> MSAEAADREAATSSRPCTPPQTCWFEFLLEESLLEKHLRKPCPDPAPVQL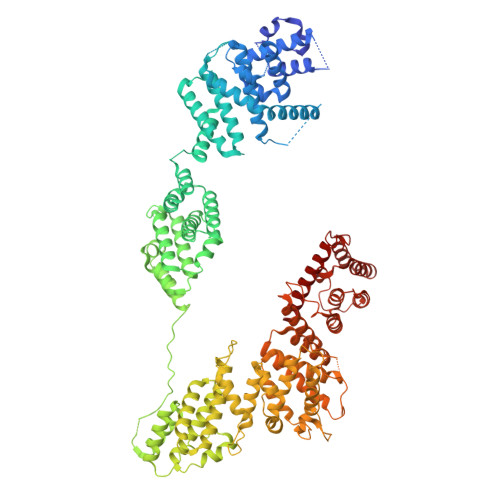IVQFLEQASKPSVNEQNQVQPPPDNKRNRILKLLALKVAAHLKWDLDILEKSLSVPVLNMLLNELLCISKVPPGTKHVDMDLATLPPTTAMAVLLYNRWAIRTIVQSSFPVKQAKPGPPQLSVMNQMQQEKELTENILKVLKEQAADSILVLEAALKLNKDLYVHTMRTLDLLAMEPGMVNGETESSTAGLKVKTEEMQCQVCYDLGAAYFQQGSTNSAVYENAREKFFRTKELIAEIGSLSLHCTIDEKRLAGYCQACDVLVPSSDSTSQQLTPYSQVHICLRSGNYQEVIQIFIEDNLTLSLPVQFRQSVLRELFKKAQQGNEALDEICFKVCACNTVRDILEGRTISVQFNQLFLRPNKEKIDFLLEVCSRSVNLEKASESLKGNMAAFLKNVCLGLEDLQYVFMISSHELFITLLKDEERKLLVDQMRKRSPRVNLCIKPVTSFYDIPASASVNIGQLEHQLILSVDPWRIRQILIELHGMTSERQFWTVSNKWEVPSVYSGVILGIKDNLTRDLVYILMAKGLHCSTVKDFSHAKQLFAACLELVTEFSPKLRQVMLNEMLLLDIHTHEAGTGQAGERPPSDLISRVRGYLEMRLPDIPLRQVIAEECVAFMLNWRENEYLTLQVPAFLLQSNPYVKLGQLLAATCKELPGPKESRRTAKDLWEVVVQICSVSSQHKRGNDGRVSLIKQRESTLGIMYRSELLSFIKKLREPLVLTIILSLFVKLHNVREDIVNDITAEHISIWPSSIPNLQSVDFEAVAITVKELVRYTLSINPNNHSWLIIQADIYFATNQYSAALHYYLQAGAVCSDFFNKAVPPDVYTDQVIKRMIKCCSLLNCHTQVAILCQFLREIDYKTAFKSLQEQNSHDAMDSYYDYIWDVTILEYLTYLHHKRGETDKRQIAIKAIGQTELNASNPEEVLQLAAQRRKKKFLQAMAKLYF> MSRNQDVFPILDLQELVICL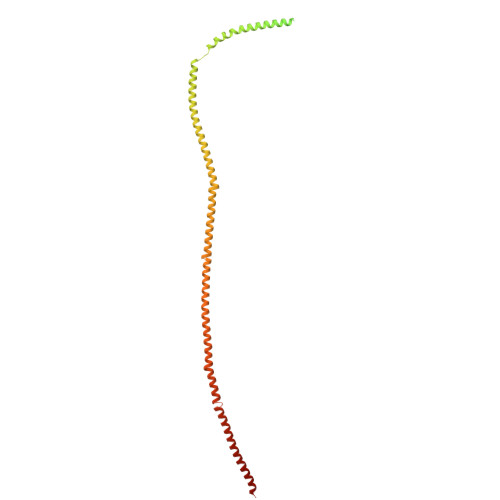QSCDFALATQENISRPTSDYMVTLYKQIIENFMGISVESLLNSSNQETGDGHLQEENENIYLDTLNVLVLNKICFKFFENIGVQDFNMTDLYKPEAQRTQRLLSAVVNYARFREERMFDCNSFILQMESLLGQLRSKFDDYNLIQQQLKQYEDVDGDNIPDEQELQKLEEQNKELEIQLKKLTKIQETLSIDYNDYKISKQSIFKDLEALSFQIVELESNRDKLIKISNTDMEELSEGIKELNDLLIQRKKTLDDLTAQQKNLQDTVTTFETIISELYDVLRIISSEVQESNRTETELVGLKQNLINNKLKLMNVLETGIMYKLEILQEQLDLQLKNLEKLSQDTKEESRLNDTKLMDLQIKYENEIKPKIDKTDIFIQEELISGKINKLNDEIKQLQKDFEVEVKEIEIEYSLLSGHINKYMNEMLEYMQ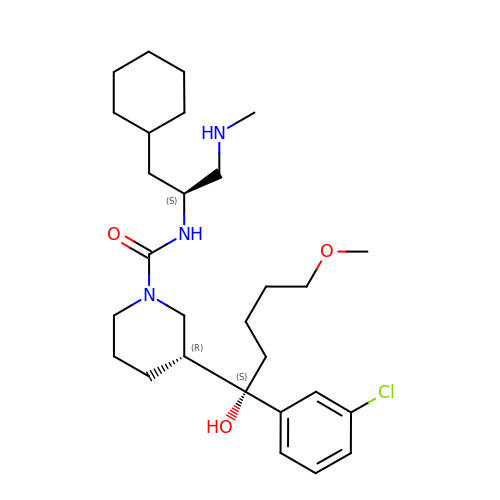(3R)-3-[(1S)-1-(3-chlorophenyl)-1-hydroxy-5-methoxypentyl]-N-{(1S)-2-cyclohexyl-1-[(methylamino)methyl]ethyl}piperidine-1-carboxamide | C28 H46 Cl N3 O3 | LGUUOHMUYOBFQP-MAARLIENSA-N> IPPIPPVDFAKYGEIEEVPMTRLMQIGATNLHRSWLN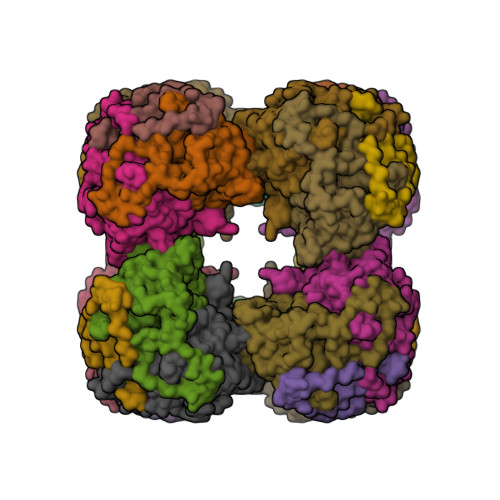VPHVTQFESADITELEAFRVAQKAVAKKAGVKLTVLPLLLKACAYLLKELPDFNSSLAPSGQALIRKKYVHIGFAVDTPDGLLVPVIRNVDQKSLLQLAAEAAELAEKARSKKLGADAMQGACFTISSLGHIGGTAFTPIVNAPEVAILGVSKASMQPVWDGKAFQPRLMLPLSLSYDHRVINGAAAARFTKRLGDLLADIRAILL The UbiD decarboxylases are prevalent in microbes and reversibly decarboxylate (hetero)aromatic and unsaturated aliphatic acid compounds using the highly modified prenylated flavin mononucleotide (prFMN) cofactor. Here, we characterize I3C decarboxylase from Arthrobacter nicotianae (AnInD). We provide structural and biochemical insights into AnInD, revealing the enzyme to be strictly specific for indole-3-carboxylic acid (I3C). Structural insights from crystal structure determination combined with small-angle X-ray scattering (SAXS) measurements reveal the enzyme undergoes an open-closed transition as a consequence of prFMN domain motion, an event likely coupled to catalysis.

AnInD structure in complex with prFMN was solved by molecular replacement. The cofactor complex structure was obtained after soaking AnInD crystals with freeze-dried prFMN powder. The AnInD structure contains an entire hexamer in the asymmetric unit. Each monomer of AnInD is composed of an N-terminal prFMN-binding domain connected to the oligomerization domain via an alpha helical linker. The C-terminal extended loop projects out and forms interactions with the prFMN-binding domain of the adjacent monomer. Electron density of bound prFMN and associated metal ions could be readily observed in the active site of the AnInD–prFMN complex structure. The phosphate moiety of the prFMN is coordinated by two metal ions, identified as Mn2+ and Na+ as these were present in the sample and by analogy to other UbiD enzymes. The prFMN-modified isoalloxazine ring is placed adjacent to the conserved E(D)-R-E network of ionic residues that is conserved in the UbiD family. A potential hinge region located on a central alpha helix (G310) can be identified, which connects the prFMN-binding domain and oligomerization domain. The crystal structure of AnInD remains poised toward the open conformation as frequently observed for other UbiDs.

>[6x]HMHKDLHSIIDALDTAGRLIRVRSQVKAEHELAGIAAKYEGCDKAVLFENVDGNDIPVLMGLYWSRDLLGSLYGVDAVDMPRFITSKISHWKSEPTAHQLIAREHAPVMAHSPRVDLLSLPIPVHAQKDGGAYVDAGVVIAADPDTGVLNTSIQRFMVENENTLHVNIDAGRHLGAYLAKAKAKGEPLSFSLNIGVHPGVHFAAATPSEVAPLDVDELGIAAEFQDGPVRIVQGDDPRVTVLADAMISLECQMYADDLADEGPFAEVTGYYAERAPRPRVTVTAVHLQRNPVFHSILSGQEVFNSVGLLGESALFDQVSKQVPGILEVALTDGGCGFYHAVVQLKQVRAGWSKQAILATFAAFPPLKMVTIVDEDVDLRNPRDVEWAMATRLDPERGILRIDDTFGHGLNPSFPDYFGSKVGFDATRSFPFEEKHERITYQDVDLSRFEIVEGHTAGGQHE> MMKILLIGMGGTIASVKGENGYEASLSVKEVLDIAGIKDCEDCDFLDLKNVDSTLIQPEDWVDLAETLYKNVKKYDGIIVTHGTDTLAYTSSMISFMLRNPPIPIVFTGSMIPATEENSDAPLNLQTAIKFATSGIRGVYVAFNGKVMLGVRTSKVRTMSRDAFESINYPIIAELRGEDLVVNFIPKFNNGEVTLDLRHDPKVLVIKLIPGLSGDIFRAAVELGYRGIVIEGYGAGGIPYRGSDLLQTIEELSKEIPIVMTTQAMYDGVDLTRYKVGRLALRAGVIPAGDMTKEAT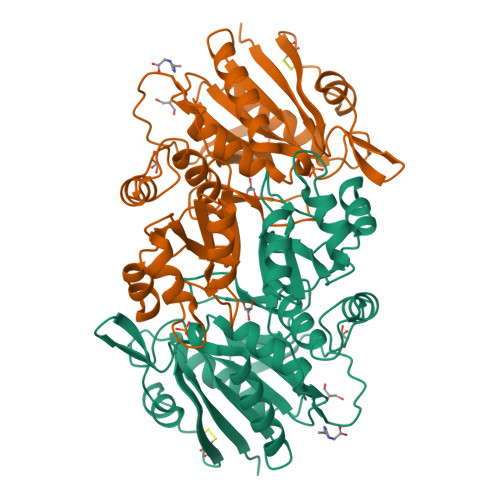VTKLMWILGHTNNVEEIKVLMRKNLVGELRD> ETNEITIGITVTTTGPAAALGIPERNALEFVAKEIGGHPLKVIVLDDGGDPTAATTNARRFVTESKADVIMGSSVTPPTVAVSNVANEAQVPHIALAPLPITPERAKWSVAMPQPIPIMGKVLYEHMKKNNIKTVGYIGYSDSYGDLWFNDLKKQGEAMGLKIVAEERFARPDTSVAGQVLKLVAANPDAILVGASGTAAALPQTSLRERGYKGLIYQTHGAASMDFIRIAGKSAEGVLMASGPVMDPEGQDDSALTKKPGLELNTAYEAKYGPNSRSQFAAHSFDAFKVLERVVPVALKTAKPGTQEFREAIRKALVSEKDIAASQGVYSFTETDRYGLDDRSRILLTVKDGKYVMVKAAALEHHHHHH

In this paper we compare the ligand specificity and binding affinities of the periplasmic binding proteins RPA1782 and RPA1789 from the TRAP and ABC systems of the non β- oxidation pathway gene cluster respectively. Data from a combination of fluorescence spectroscopy and ITC clearly show that both proteins have binding affinities in the nanomolar range for coumarate, caffeate and ferulate, with weaker (but still high affinity) binding of cinnamate. In view of the tight binding of coumarate to RPA1789 evidenced by both ITC and fluorescence spectroscopy, the genome context of the rpa1789 and rpa1791-1793 transporter genes, their clustering with coumarate catabolic genes and their common regulation by CouR, we propose that the components of this ABC transporter be designated CouP (RPA1789), CouS (RPA1791), CouT (RPA1792) and CouU (RPA1793). The structure displays all the features expected of an ABC-bacterial periplasmic binding protein; namely a two-domain structure in which an intrinsic cleft positioned between the two domains forms the ligand-binding pocket.

After a denaturation and refolding protocol that removed this endogenous ligand contaminant, a 2.5 Å structure with coumarate bound and a 1.9 Å structure with ferulate bound were determined. Thus, we will not discuss its structure further here, other than to note that the mode of ligand binding is identical to that for ferulate. A summary of the relevant data processing and refinement statistics for the ferulate complex and the ligand free form are presented in Table 3, and the 1.9 Å structure of CouP with ferulate bound is shown in Figure 5. Analysis of the interactions in the binding cleft show that the aromatic ring of the ligand is bound most deeply. Key H-bond interactions are formed between the 4-OH group of the aromatic ring of ferulate with His309 and Gln305 residues. H-bond interactions are also made between the carboxyl group on the ferulate side chain and Arg197, Ser222 and Thr102. These latter interactions explain why compounds such as 4-hydroxybenzoate showed no evidence of binding; they lack the 3-carbon chain that ensures optimal bond distances on each side of the binding cleft are formed. The methoxy-group possessed by ferulate sits in a pocket bounded by the side chains of Leu46, Phe306 and His309 and the main chain carbonyl oxygen atoms of Ser100 and Leu122. There are also close ligand contacts with Glu50, Phe306 and His309. The data also explain how structurally similar ligand contaminants like 4-HPP can be incorporated into the binding pocket.> GSHMAATAAEAVASGSGEPREEAGALGPAWDESQLRSYSFPTRPIPRLSQSDPRAEELIENEEPVVLTDTNLVYPALKWDLEYLQE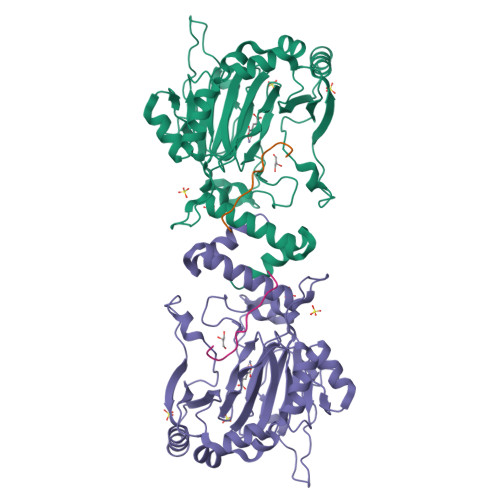NIGNGDFSVYSASTHKFLYYDEKKMANFQNFKPRSNREEMKFHEFVEKLQDIQQRGGEERLYLQQTLNDTVGRKIVMDFLGFNWNWINKQQGKRGWGQLTSNLLLIGMEGNVTPAHYEEQQNFFAQIKGYKRCILFPPDQFECLYPYPVHHPCDRQSQVDFDNPDYERFPNFQNVVGYETVVGPGDVLYIPMYWWHHIESLLNGGITITVNFWYKGAPTPKRIEYPLKAHQKVAIMRNIEKMLGEALGNPQEVGPLLNTMIKGRYN;> DESGLPQLTSYDAEVNAPI> VGG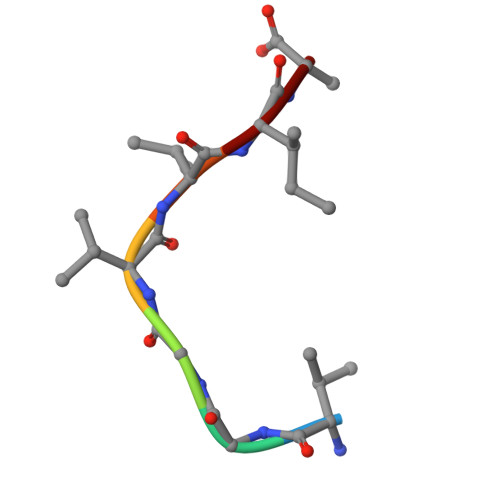VVIA> MPITIGNGFLKSEILTNSPRNTKEAWWKVLWEKIKDFFFSTGKAKADRCLHEMLFAERAPTRERLTEIFFELKELACASQRDRFQVHNPHENDATIILRIMDQNEENELLRITQNTDTFSCEVMGNLYFLMKDRPDILKSHPQMTAMIKRRYSE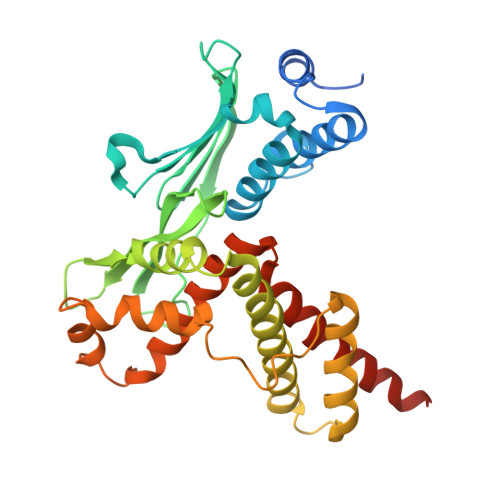IVDYPLPSTLCLNPAGAPILSVPLDNIEGYLYTELRKGHLDGWKAQEKATYLAAKIQSGIEKTTRILHHANISESTQQNAFLETMAMCGLKQLEIPPPHTHIPIEKMVKEVLLADKTFQAFLVTDPSTSQSMLAEIVEAISDQVFHAIFRIDPQAIQKMAEEQLTTLHVRSEQQSGCLCCFL N-(2,6-diethylphenyl)-N'-(N-propylcarbamimidoyl)urea 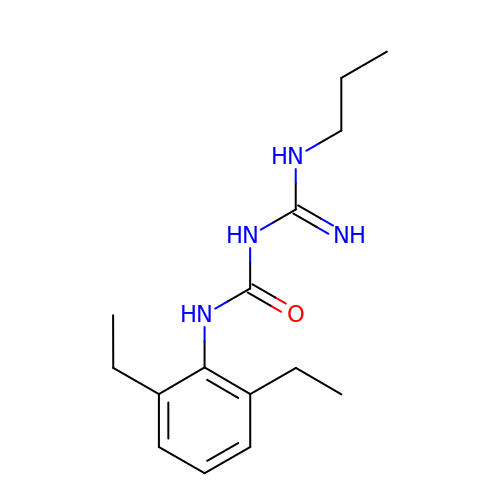| C15 H24 N4 O | DWPYTUBIBPCLBG-UHFFFAOYSA-N> GPGSMMDHLHATPGMFVQHSTAIFSDRYKGQRVLGKGSFGEVILCKDKITGQECAVKVISKRQVKQKTDKESLLREVQLLKQLDHPNIMKLYEFFEDKGYFYLVGEVYTGGELFDEIISRKRFSEVDAARIIRQVLSGITYMHKNKIVHRDLKPENLLLESKSKDANIRIIDFGLSTHFEASKKMKDKIGTAYYIAPEVLHGTYDEKCDVWSTGVILYILLSGCPPFNGANEYDILKKVEKGKYTFELPQWKKVSESAKDLIRKMLTYVPSMRISAR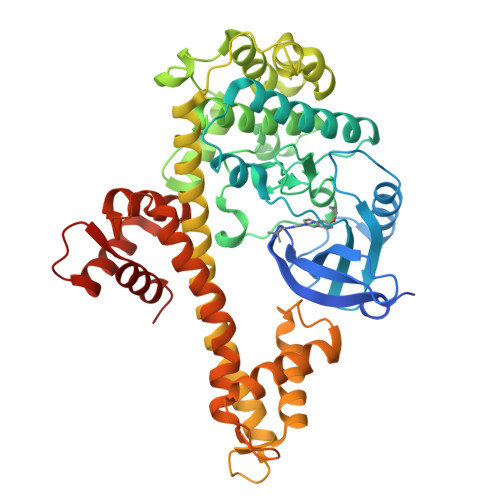DALDHEWIQTYTKEQISVDVPSLDNAILNIRQFQGTQKLAQAALLYMGSKLTSQDETKELTAIFHKMDKNGDGQLDRAELIEGYKELMRMKGQDASMLDASAVEHEVDQVLDAVDFDKNGYIEYSEFVTVAMDRKTLLSRERLERAFRMFDSDNSGKISSTELATIFGVSDVDSETWKSVLSEVDKNNDGEVDFDEFQQMLLKLCGN> GVS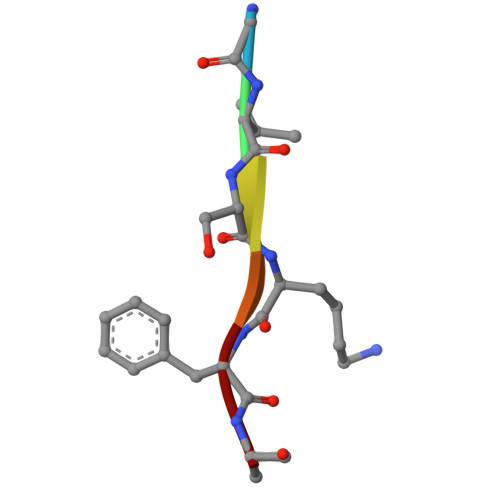KFA>MRMSDGAAPKANGSEASGQDLVPTAVEQAVPIQPVAGSALAAPAAGQINQIDPWIFQNFVQCPLGEFSISPRNTPGEILFDLALGPGLNPYLAHLSAMYTGWVGNMEVQLVLAGNAFTAGKVVVALVPPYFPKGSLTTAQITCFPHVMCDVRTLEPIQLPLLDVRRVLWHATQDQEESMRLVCMLYTPLRTNSPGDESFVVSGRLLSKPAADFNFVYLTPPIERTIYRMVDLPVLQPRLCTHARWPAPIYGLLVDPSLPSNPQWQNGRVHVDGTLLGTTPVSGSWVSCFAAEAAYEFQSGTGEVATFTLIEQDGSAYVPGDRAAPLGYPDFSGQLEIEVQTETTKTGDKLKVTTFEMILGPTTNVDQAPYQGRVYASLTAVASLDLVDGRVRAVPRSIYGFQDVIPEYNDGLLVPLAPPIGPFLPGEVLLRFRTYMRQLDTADAAAEAIDCALPQEFISWFASNAFTVQSDALLLRYRNTLTGQLLFECKLYSEGYIALSYSGSGPLTFPTDGFFEVVSWVPRLFQLASVGSLTTGRTLKQ[2x];> MHLSLLVPFLFWITGCCTAEDPVTGPEEVSGQEQGSLTVQCRYTSGWKDYKKYWCQGVPQRSCKTLVETDASEQLVKKNRVSIRDNQRDFIFTVTMEDLRMSDAGIYWCGITKGGLDPMFKVTVNIGPVPTMPPITSTTTIFTVTTTVKETSMFPTLTSYYSDNGHGGGDSGGGEDGVGDGFLDLSVLLPVISAVLLLLLLVASLFAWRMVRRQKKAAGPPSEQAQSLEGDLCYADLSLKQPRTSPGSSWKKGSSMSSSGKDHQEEVEYVTMAPFPREEVSYAALTLAGLGQEPTYGNTG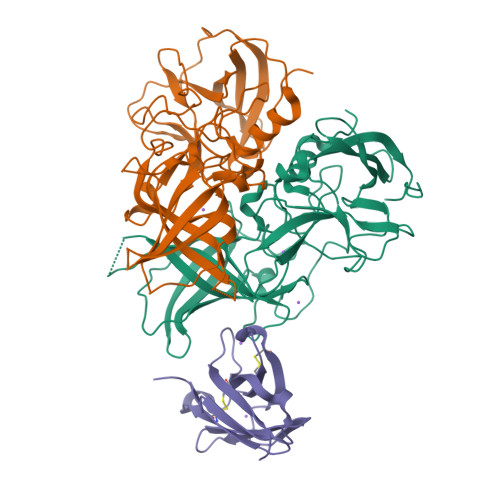CPITHVPRTGLEEETTEYSSIRRPLPAAMP1-isoquinolin-6-yl-3-[2-oxo-2-(pyrrolidin-1-yl)ethyl]urea 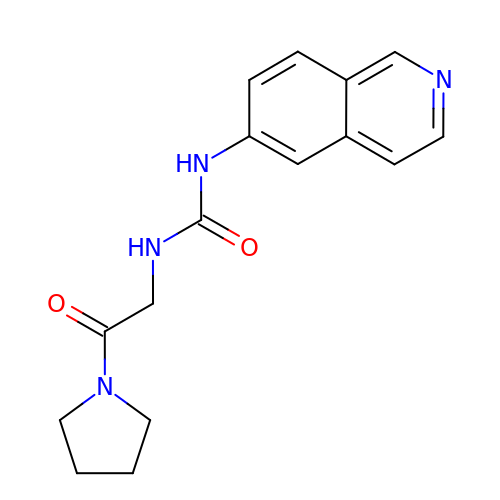| C16 H18 N4 O2 | DMIDPTCQPIJYFE-UHFFFAOYSA-N7-METHYL-6-THIO-GUANOSINE | 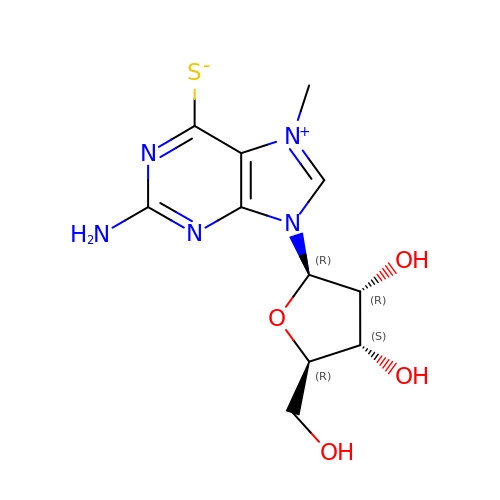C11 H15 N5 O4 S | RFHIWBUKNJIBSE-KQYNXXCUSA-N In Gram-negative bacteria, the full Dpp transporter is composed of five subunits: two integral membrane proteins (DppB and DppC) that form a translocation pathway for substrates; two ATPases (DppD and DppF) that bind and hydrolyze ATP during transport and a periplasm-localized SBP (DppA) for substrate capture. The Dpp transporter is primarily responsible for importing dipeptides but also capable of inefficiently importing tri- and tetrapeptides into the cell. Different from those structurally and mechanistically well-characterized ABC exporters that solely consist of two variable transmembrane domains (TMDs) and two highly conserved nucleotide-binding domains (NBDs), the ABC peptide importers require an additional substrate-binding protein (SBP) that captures peptide substrates and delivers them to the translocator for function. Unlike the reported heterotrimeric Mycobacterium tuberculosis DppBCD translocator, the E. coli DppBCDF translocator is a heterotetramer, with a [4Fe-4S] cluster at the C-terminus of each ATPase subunit.

Using this strategy, we determined the ATPγS-bound DppABCDE179QFE187Q complex structure at 2.73 Å by addition of ATPγS and Mg2+ prior to cryo-EM sample preparation, and we refer to this structure as ATPγS-DppABCDF unless otherwise specified. Structure reveals that DppABCDF forms a compact pentameric structure with an approximate dimension of 70 × 70 × 140 Å. A DppA molecule caps at the top of the two integral membrane proteins, DppB and DppC, in the periplasm, and two ATPases, DppD and DppF, adopt a closed conformation in the cytosol. Unlike apo-DppBCDF and ATPγS (or AMPPNP)-DppBCDF, which adopt an inward-facing conformation, ATPγS-DppABCDF adopts an outward-facing conformation with two ATPγS molecules bound at the interface of the two NBDs. In ATPγS-DppABCDF, a striking rearrangement of the TM helices of both DppB and DppC, which form the substrate translocation pathway, results in the opening of the periplasmic substrate entry gate. Specifically, the periplasmic substrate entry gate is open to approximately 9.0 Å in diameter in ATPγS-DppABCDF. The two ATPγS molecules act as molecular glues, shortening the Cα–Cα distance between the D-loop T182DppD and the opposite D-loop S190DppF in the RecA-like subdomain from 10.4 to 5.6 Å. However, in ATPγS-DppABCDF, the DppB scoop motif, which consists of two short α helices (α1 and α2) connected by a scoop loop, is clearly resolved. In particular, its α1 helix and α2 helix interact with the C-lobe and the N-lobe of DppA, respectively, whereas the side chains of two conserved charged residues, E41DppB and R42DppB, from the scoop loop form two salt bridges with side chains of residues R383DppA and D436DppA. Taken together, these findings suggest that concurrent binding of DppA and ATP to DppBCDF does induce conformational changes of translocator, and the ATPγS-DppABCDF structure snapshots a typical pre-catalytic (or ATP-bound) state of the transporter.

> MLQFILRRLGLVIPTFIGITLLTFAFVHMIPGDPVMIMAGERGISPERHAQLLAELGLDKPMWQQYLHYIWGVMHGDLGISMKSRIPVWEEFVPRFQATLELGVCAMIFATAVGIPVGVLAAVKRGSIFDHTAVGLALTGYSMPIFWWGMMLIMLVSVHWNLTPVSGRVSDMVFLDDSNPLTGFMLIDTAIWGEDGNFIDAVAHMILPAIVLGTIPLAVIVRMTRSSMLEVLGEDYIRTARAKGLTRMRVIIVHALRNAMLPVVTVIGLQVGTLLAGAILTETIFSWPGLGRWLIDALQRRDYPVVQGGVLLVATMIILVNLLVDLLYGVVNPRIRHKK;> MSQVTENKVISAPVPMTPLQEFWHYFKRNKGAVVGLVYVVIVLFIAIFANWIAPYNPAEQFRDALLAPPAWQEGGSMAHLLGTDDVGRDVLSRLMYGARLSLLVGCLVVVLSLIMGVILGLIAGYFGGLVDNIIMRVVDIMLALPSLLLALVLVAIFGPSIGNAALALTFVALPHYVRLTRAAVLVEVNRDYVTASRVAGAGAMRQMFINIFPNCLAPLIVQASLGFSNAILDMAALGFLGMGAQPPTPEWGTMLSDVLQFAQSAWWVVTFPGLAILLTVALFNLMGDGLRDALDPKLKQ;> MALLNVDKLSVHFGDESAPFRAVDRISYSVKQGEVVGIVGESGSGKSVSSLAIMGLIDYPGRVMAEKLEFNGQDLQRISEKERRNLVGAEVAMIFQDPMTSLNPCYTVGFQIMEAIKVHQGGNKSTRRQRAIDLLNQVGIPDPASRLDVYPHQLSGGMSQRVMIAMAIACRPKLLIADQPTTALDVTIQAQIIELLLELQQKENMALVLITHDLALVAEAAHKIIVMYAGQVVETGDAHAIFHAPRHPYTQALLRALPEFAQDKERLASLPGVVPGKYDRPNGCLLNPRCPYATDRCRAEEPALNMLADGRQSKCHYPLDDAGRPTL;> MSTQEATLQQPLLQAIDLKKHYPVKKGMFAPERLVKALDGVSFNLERGKTLAVVGESGCGKSTLGRLLTMIEMPTGGELYYQGQDLLKHDPQAQKLRRQKIQIVFQNPYGSLNPRKKVGQILEEPLLINTSLSKEQRREKALSMMAKVGLKTEHYDRYPHMFSGGQRQRIAIARGLMLDPDVVIADQPVSALDVSVRAQVLNLMMDLQQELGLSYVFISHDLSVVEHIADEVMVMYLGRCVEKGTKDQIFNNPRHPYTQALLSATPRLNPDDRRERIKLSGELPSPLNPPPGCAFNARCRRRFGPCTQLQPQLKDYGGQLVACFAVDQDENPQR;> MRISLKKSGMLKLGLSLVAMTVAASVQAKTLVYCSEGSPEGFNPQLFTSGTTYDASSVPLYNRLVEFKIGTTEVIPGLAEKWEVSEDGKTYTFHLRKGVKWHDNKEFKPTRELNADDVVFSFDRQKNAQNPYHKVSGGSYEYFEGMGLPELISEVKKVDDNTVQFVLTRPEAPFLADLAMDFASILSKEYADAMMKAGTPEKLDLNPIGTGPFQLQQYQKDSRIRYKAFDGYWGTKPQIDTLVFSITPDASVRYAKLQKNECQVMPYPNPADIARMKQDKSINLMEMPGLNVGYLSYNVQKKPLDDVKVRQALTYAVNKDAIIKAVYQGAGVSAKNLIPPTMWGYNDDVQDYTYDPEKAKALLKEAGLEKGFSIDLWAMPVQRPYNPNARRMAEMIQADWAKVGVQAKIVTYEWGEYLKRAKDGEHQTVMMGWTGDNGDPDNFFATLFSCAASEQGSNYSKWCYKPFEDLIQPARATDDHNKRVELYKQAQVVMHDQAPALIIAHSTVFEPVRKEVKGYVVDPLGKHHFENVSIE> MFAKQIDIHWQKMKGIKFLHWLLGTVLLWVSLSTPALAIPALDYNPWEAIQLPTTATILDMSFIDRHHGWLVGVNATLMETRDGGQTWEPRTLVLDHSDYRFNSVSFQGNEGWIVGEPPIMLHTTDGGQSWSQIPLDPKLPGSPRLIKALGNGSAEMITNVGAIYRTKDSGKNWQALVQEAIGVMRNLNRSPSGEYVAVSSRGSFYSTWEPGQTAWEPHNRTTSRRLHNMGFTPDGRLWMIVNGGKIAFS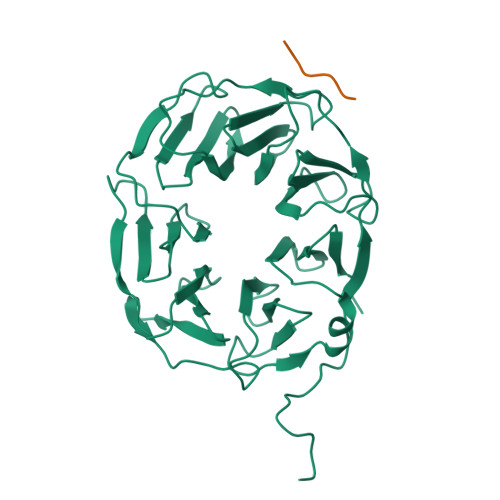DPDNSENWGELLSPLRRNSVGFLDLAYRTPNEVWLAGGAGALLCSQDGGQTWQQDVDVKKVPSNFYKILFFSPDQGFILGQKGILLRYVTDLTAAPA;> NAHNFPLDLA>HMLTIRLLMHGKEVGSIIGKKGESVKRIREESGARINISEGNSPERIITLTGPT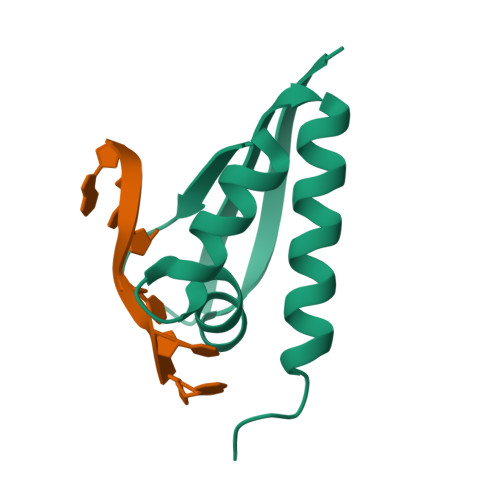NAIFKAFAMIIDKLEEDINSSW[4x]> KGHLTRLGLEFFDQPAVPLARAFLGQVLVRRLPNGTELRGRIVETQAYLGPEDEAAHSRGGRQTPRNRGMFMKPGTLYVYIIYGMYFC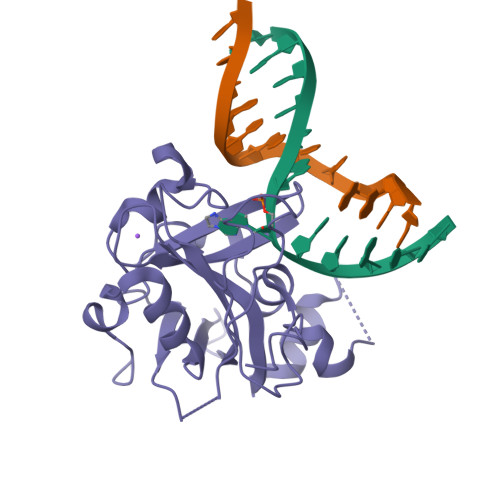MNISSQGDGACVLLRALEPLEGLETMRQLRSTLRKGTASRVLKDRELCSGPSKLCQALAINKSFDQRDLAQDEAVWLERGPLEPSEPAVVAAARVGVGHAGEWARKPLRFYVRGSPWVSVVDRVAEQDTQA>[2x]GKQEELKRLHRAQIIQRQLQQV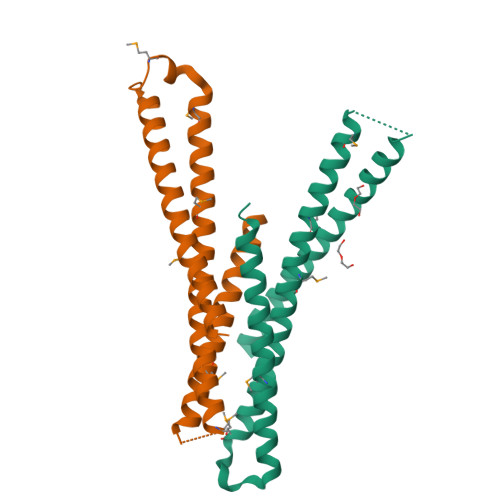EERQRRLEERGVAVEKALRGEAGMGKKDDPKLMQEWFKLVQEKNAMVRYESELMIFARELELEDRQSRLQQELRERMAVEDHLKTEEELSEEKQILNEMLEVVEQRDSLVALLEEQRLREREEDKDLEA>[8x]MIFMRKVVA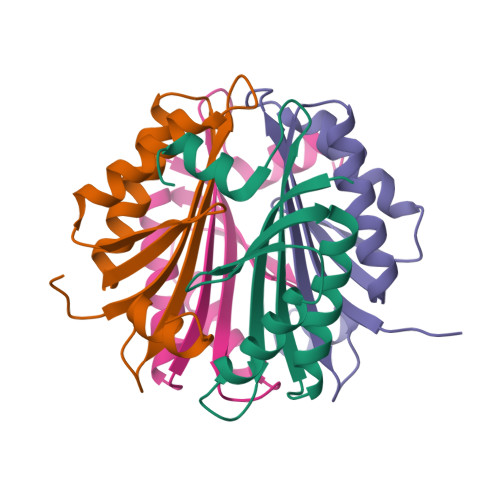EVSIIPLGKGASVSKYVKKAIEVFKKYDLKVETNAMGTVLEGDLDEILKAFKEAHSTVLNDVDRVVSSLKIDERKDKENTIERKLKAIGEL(1S,3R,4S,5R)-1,3,4,5-tetrahydroxycyclohexanecarboxylic 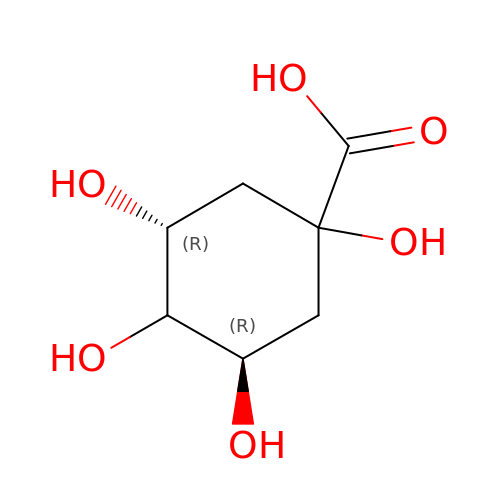acid | C7 H12 O6 | AAWZDTNXLSGCEK-WYWMIBKRSA-N> ATFEIVNRCSYTVWAAASKGDAALDAGGRQLNSGESWTINVEPGTNGGKIWARTDCYFDDSGSGICKTGDCGGLLRCKRFGRPPTTLAEFSLNQYGKDYIDISNIKGFNVPMNFSPTTRGCRGVRCAADIVGQCPAKLKAPGGGCNDACTVFQTSEYCCTTGKCGPTEYSRFFKRLCPDAFSYVLDKPTTVTCPGSSNYRVTFCPTA

The helium path was used for collection of anomalous diffraction data at 5 keV for two proteins: thaumatin and the membrane protein TehA. Although anomalous signals from each individual crystal are very weak, robust anomalous signals are obtained from data assembled from micrometre-sized crystals. The thaumatin structure was determined from 15 microcrystals and the TehA structure from 18 microcrystals. These results demonstrate the usefulness of a helium environment in support of native-SAD phasing at 5 keV.

Thaumatin consists of 207 residues, including 1 me­thio­nine and 16 cysteines forming 8 di­sulfide bridges. The calculated Bijvoet difference ratio is 2.8% at 5 keV. We collected a total of 17 datasets with the helium path, each from a single crystal. Individually, none of them showed significant anomalous signals. We performed native-SAD phasing for the 15-crystal dataset. With an E min cutoff at 1.3 and resolution cutoff at 3.9 Å, we obtained a substructure solution including 9 sulfur peaks from as few as 80 SHELXD trials with the highest CCall and CCweak of 48.6 and 28.7%, respectively [Fig. 3(a)]. BUCCANEER was able to build 206 out of 207 residues automatically. The refined structure has an R/R free of 0.19/0.23, indicating high quality [Fig. 3(c)].Mitochondrial poration by pore-forming BCL-2 Effectors, BAK and BAX, initiates apoptosis. BAK is dormant in healthy cells. Its apo structure exhibits a stable globular conformation incapable of executing poration. Autoactivation is mechanistically similar to direct activation: binding of exposed BH3 of BAK or activators to the activation groove induces conformational changes in the electrostatic network at the bottom of this groove destabilizing helix α1 to initiate BAK unfolding.

Here we show that autoactivation involves binding in trans of the BH3 helix α2 of active BAK to the activation groove of dormant BAK. To stabilize and crystallize autoactivated BAK, we disulfide-tethered BAK BH3GGC peptide to engineered G184C BAK (herein referred to as BAK BH3-BAK complex). We determined the crystal structure of this complex to 3.1 Å resolution, which revealed 10 unique complexes in the asymmetric unit. Cu2+ acts as crystal contact coordinating two BAK monomers. The GGC linker is largely invisible in all 10 complexes suggesting its intrinsic disorder and minimal contribution to the structure of the complex beyond tethering. The BAK BH3 peptide forms a helix bound to the activation groove of BAK, similar to previous BH3-bound complexes of BAK. However, in marked contrast to those previous BAK complexes, autoactivated BAK exhibits rearrangements of a buried electrostatic network with helix α1 at the bottom of the activation groove. In apo BAK helix α1 electrostatic network is stabilized by 2 hydrogen bonds between α1 R42 and α3 D90 and 2 hydrogen bonds between α1 E46 and α5 R137. Of the 10 autoactivated BAK here, seven feature 2 hydrogen bonds between α1 R42 and E46 and α2 N86; one has only 1 hydrogen bond between α1 R42 and α2 N86; and two (those with lowest b-factors) show no visible density for this network. The destabilized conformation of the electrostatic network is unique to autoactivated BAK providing the structural basis of BAK triggering by BAK BH3.

>SASEEQVAQDTEEVFRSYVFYRHQQEQEAEGVAAPADPEMVTLPLQPSSTMGQVGRQLAIIGDDINRRYDSEFQTMLQHLQPTAENAYEYFTKIATSLFESGINWGRVVALLGFGYRLALHVYQHGLTGFLGQVTRFVVDFMLHHSIARWIAQRGGWVAALNLCNG[10x];>[10x]SSTMGQVGRQLAIIGDDINRRYGGC>[4x]QNPQQLSANLWAAVRARGCQFLGPAMQE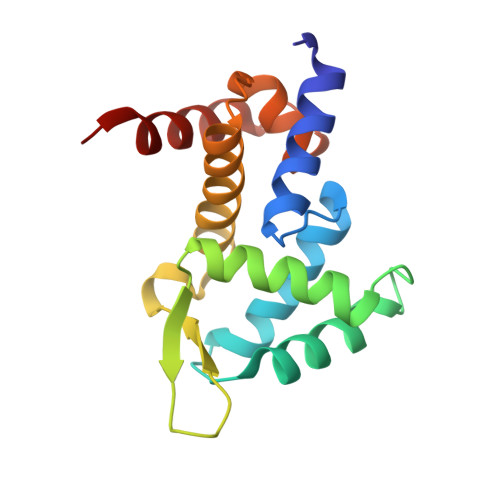EALKLVLLALEDGSALSRKVLVLFVVQRLEPRFPQASKTSIGHVVQLLYRASCFKVTKRDEDSSLMQLKEEFRSYEALRREHDAQIVHIAMEAGLRISPEQWSSLLYGDLAHKSHMQSIIDKLQSPE> ATLAQDVIDRFDVSRPELYRDDLWQAPFRELRATAPVHRVEHSDFGPYWSVSSYKPIITVESLPDLYSSAGGITLADFIENNPTDVRMPMFIAMDRPKHTGQRRTVAPAFTPSEMVRMSDNIRMRTAEVLDSLEWNTPFDWVDTVSVELTTQMLAILFDFPWEERRKLTFWSDWAGDIELVKNEELRLERLRHMYECGGYFQNLWNAKIGKPPTPDLISMMIHSDAMAEMDQMEFLGNLILLIVGGNDTTRNTMSAVAYGLDLFPDQRAKLEADPSMIPNTVQEIIRWQTPLAHMRRTATVDSELEGQQIKAGDKLALWYISANRDESVFENADRIIVDRPNARRHLAFGHGIHRCVGARLAELQIAVLLEEMAKRRMRVNVLGEPERVAACFVHGYRKLPVEISRY

Cytochrome P450 enzymes (CYPs) are heme-containing proteins that catalyze the insertion of oxygen into a wide variety of substrates. In the current study, we evaluated CYP153D17 (NCBI Reference Sequence, WP_010183267.1) from the endosymbiotic bacterium Sphingomonas sp. strain PAMC 26605. Sequence analysis revealed that CYP153D17 has 48.27% identity with P450pyr hydroxylase from Sphingopyxis macrogoltabida and that it contains conserved motifs including an oxygen-binding domain and heme-binding domains found in typical CYPs. In this study, we identified CYP153D17 from the endosymbiotic bacterium Sphingomonas sp. PAMC 26605 as a putative alkane-hydroxylating cytochrome P450 enzyme based on our substrate binding assay and structural data.

In addition, we determined the crystal structure of CYP153D17 at 3.1 Å resolution in complex with a co-purified alkane-like compound. The structure was refined to a resolution of 3.1 Å and had a typical CYP fold, comprising a central heme molecule surrounded by 13 α-helices and 7 β-strands. The putative substrate-binding pocket of CYP153D17 was found to be shaped similar to a cone funnel with a length and outer diameter of approximately 17 and 10 Å, respectively. Notably, an additional electron density map appeared within the substrate-binding pocket during refinement. Because exogenous ligands were not added to the crystallization solutions, the bound molecule may have co-purified with the enzyme during the production of recombinant protein. Substrate binding assay data suggested that the ligand was an alkane-like compound and the electron density was modeled as dodecane. The co-purified ligand was bound to the hydrophobic substrate-binding pocket created by the Met90, Ala175, Ile240, Leu241, Val244, Leu292, Met295, and Phe393 residues. The overall protein structure of P450pyr (best hit in the DALI search) was very similar to that of CYP153D17 (r.m.s. deviation, 0.96 Å for 307 Cα atoms), but P450pyr contained no ligand and the loop region (residues 88–96 in P450pyr) between the α3 and α4-helix was missing in the P450pyr structure. Structural superposition revealed that the binding mode of phytanic acid was similar to that of the co-purified ligand of CYP153D17 as an extended conformation. Therefore, it is expected that for CYP153D17, hydroxylation may also be performed at the end of alkane molecules, such as in CYP124-mediated ω-oxidation.>[3x]GPGSGAYVYRSAFSVGLETYVTIPNMPIRFTKIFYNQQNHYDGSTGKFHCNIPGLYYFAYHITVYMKDVKVSLFKKD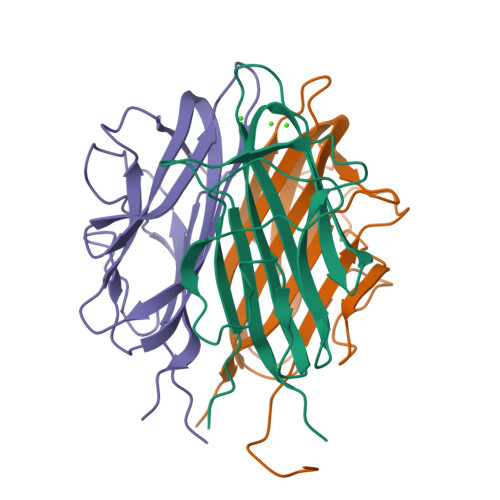KAMLFTYDQYQENNVDQASGSVLLHLEVGDQVWLQVYGEGERNGLYADNDNDSTFTGFLLYHDTN>[2x]H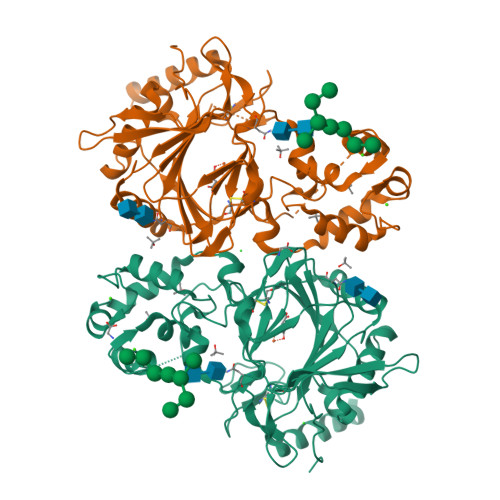HHHHHDESSDPGPQHRVQGPGPEPTLGPLTRLEGIKVGHERKVQLVTDRDHFIRTLSLKPLLFEIPGFLTDEECRLIIHLAQMKGLQRSQILPTEEYEEAMSTMQVSQLDLFRLLDQNRDGHLQLREVLAQTRLGNGWWMTPESIQEMYAAIKADPDGDGVLSLQEFSNMDLRDFHKYMRSHKAESSELVRNSHHTWLYQGEGAHHIMRAIRQRVLRLTRLSPEIVELSEPLQVVRYGEGGHYHAHVDSGPVYPETICSHTKLVANESVPFETSCRYMTVLFYLNNVTGGGETVFPVADNRTYDEMSLIQDDVDLRDTRRHCDKGNLRVKPQQGTAVFWYNYLPDGQGWVGDVDDYSLHGGCLVTRGTKWIANNWINVDPSRARQALFQQEMARLAREGGTDSQPEWALDRAYRDARVEL> MNDDRETPPKRKPGEDDTLFDIDFLDDTTSHSGSRSKVTNSHANANYI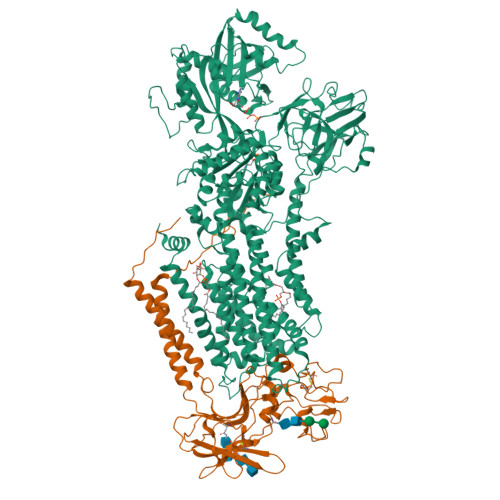PPSHVLPEETIDLDADDDNIENDVHENLFMSNNHDDQTSWNANRFDSDAYQPQSLRAVKPPGLFARFGNGLKNAFTFKRKKGPESFEMNHYNAVTNNELDDNYLDSRNKFNIKILFNRYILRKNVGDAEGNGEPRVIHINDSLANSSFGYSDNHISTTKYNFATFLPKFLFQEFSKYANLFFLCTSAIQQVPHVSPTNRYTTIGTLLVVLIVSAMKECIEDIKRANSDKELNNSTAEIFSEAHDDFVEKRWIDIRVGDIIRVKSEEPIPADTIILSSSEPEGLCYIETANLDGETNLKIKQSRVETAKFIDVKTLKNMNGKVVSEQPNSSLYTYEGTMTLNDRQIPLSPDQMILRGATLRNTAWIFGLVIFTGHETKLLRNATATPIKRTAVEKIINRQIIALFTVLIVLILISSIGNVIMSTADAKHLSYLYLEGTNKAGLFFKDFLTFWILFSNLVPISLFVTVELIKYYQAFMIGSDLDLYYEKTDTPTVVRTSSLVEELGQIEYIFSDKTGTLTRNIMEFKSCSIAGHCYIDKIPEDKTATVEDGIEVGYRKFDDLKKKLNDPSDEDSPIINDFLTLLATCHTVIPEFQSDGSIKYQAASPDEGALVQGGADLGYKFIIRKPNSVTVLLEETGEEKEYQLLNICEFNSTRKRMSAIFRFPDGSIKLFCKGADTVILERLDDEANQYVEATMRHLEDYASEGLRTLCLAMRDISEGEYEEWNSIYNEAATTLDNRAEKLDEAANLIEKNLILIGATAIEDKLQDGVPETIHTLQEAGIKIWVLTGDRQETAINIGMSCRLLSEDMNLLIINEETRDDTERNLLEKINALNEHQLSTHDMNTLALVIDGKSLGFALEPELEDYLLTVAKLCKAVICCRVSPLQKALVVKMVKRKSSSLLLAIGDGANDVSMIQAAHVGVGISGMEGMQAARSADIAVGQFKFLKKLLLVHGSWSYQRISVAILYSFYKNTALYMTQFWYVFANAFSGQSIMESWTMSFYNLFFTVWPPFVIGVFDQFVSSRLLERYPQLYKLGQKGQFFSVYIFWGWIINGFFHSAIVFIGTILIYRYGFALNMHGELADHWSWGVTVYTTSVIIVLGKAALVTNQWTKFTLIAIPGSLLFWLIFFPIYASIFPHANISREYYGVVKHTYGSGVFWLTLIVLPIFALVRDFLWKYYKRMYEPETYHVIQEMQKYNISDSRPHVQQFQNAIRKVRQVQRMKKQRGFAFSQAEEGGQEKIVRMYDTTQKRGKYGELQDASANPFNDNNGLGSNDFESAEPFIENPFADGNQNSNRFSSSRDDISFDI;> MVSLFKRGKAPPLTKEGPTSKKPPNTAFRQQRLKAWQPILSPQSVLPLLIFVACIFTPIGIGLIVSATKVQDLTIDYSHCDTKASTTAFEDIPKKYIKYHFKSKVENKPQWRLTENENGEQSCELQFEIPNDIKKSIFIYYKITNFYQNHRRYVQSFDTKQILGEPIKKDDLDTSCSPIRSREDKIIYPCGLIANSMFNDTFSQVLSGIDDTEDYNLTNKHISWSIDRHRFKTTKYNASDIVPPPNWMKKYPDGYTDENLPDIHTWEEFQVWMRTAAFPKFYKLTLKNESASLPKGKYQMNIELNYPISLFGGTKSFVLTTNGAIGGRNMSLGVLYLIVAGLCALFGIIFLVKLIFQPRAMGDHTYLNFDDEENEDYEDVHAENTTLREIL> MTRRLRVHNGVEDDLFEAFSYYADAAPDQIDRLYNLFVDAVTKRIPQAPNAFAPLFKHYRHIYLRPFRYYVAYRTTDEAIDILAVRHGMENPNAVEAEISGRTFE;> MVVNRALLASVDALSRDEQIELVEHINGNLAEGMHISEANQALIEARANDTDDAHWSTIDDFDKRIRARLG

The widespread and highly conserved ParDE TA systems, part of the RelE/ParE superfamily, target DNA gyrase. M. tuberculosis encodes two ParDE systems and several studies on the ParE1 and ParE2 toxins have shown their ability to inhibit gyrase enzymes from E. coli, M. smegmatis and M. tuberculosis. Toxin-antitoxin (TA) systems are found in most bacterial genomes and generally comprise small bicistronic loci encoding a protein toxin and a protein or RNA antitoxin. Here, we present microbiological, biochemical, structural and biophysical characterisation of the ParDE1 and ParDE2 TA systems from M. tuberculosis.

The ParDE2 crystal structure exists as a heterodimer containing a half-unresolved ParD2 antitoxin. The ParE2 toxin is comprised of β1 (R4–H8), α1 (N9–Y22), α2 (P27–Q47), β2 (R60–Y63), β3 (Y69–T75), β4 (A79–H87), with the C-terminal M88–E105 being unresolved. β1/α1 and α2 form a hairpin structure which links to the anti-parallel β sheet core of β2–β4. The ParD2 antitoxin is comprised of α1 (E38–N49), α2 (D53–H55), α3 (I59–R69), with the N-terminal V2–H35 being unresolved in the crystal structure. A RelE/ParE superfamily alignment allowed us to plot and visualise the conserved hydrophobic residues within the ParE2 toxin structure, which are clearly concentrated on the internally facing residues of the α helical hairpin and throughout the β sheet core of the toxin. This positioning creates two major hydrophobic grooves on the surface of the ParE2 toxin which run along the β sheet core and through to the underside of the toxin between the hairpin helices. Representing the ParD2 antitoxin alongside a surface rendered ParE2 toxin clearly demonstrates the specific interaction at the conserved hydrophobic patches, as they align closely to the truncated region of ParD2. Notable contacts are the ionic bonds formed between ParD2 E45 (on α1) and ParE2 K57 (found on the loop region between α2 and β2) and between ParD2 R47 (on α1) and ParE2 (D14) (on α1, also). In contrast, when the C-terminal helix of ParE2 is removed from the search model, unmodelled electron density is present in its place, and can be more successfully built as residues I36–N49 of ParD2. This demonstrated that ParD2 α1 displaced the predicted ParE2 α4, which likely became disordered as is seen for other ParDE system complexes. Finally, given the time taken to crystallise, and that there is no remaining space in the crystal due to packing, it was considered likely that ParDE2 underwent limited proteolysis during crystallisation. The full ParDE2 complex structure is yet to be fully elucidated as the N-terminal dimerisation domain of ParD2 was cleaved during crystallisation.> MIKQ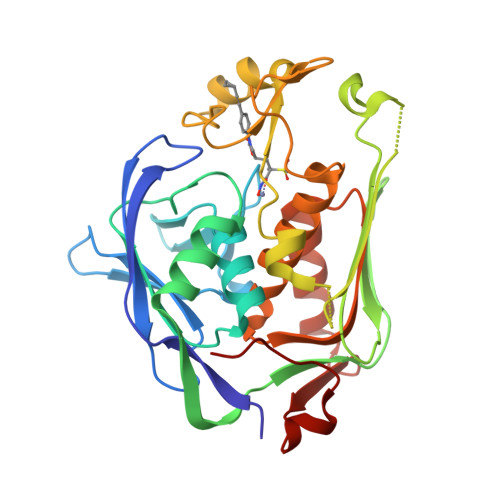RTLKNIIRATGVGLHSGEKVYLTLKPAPVDTGIVFCRTDLDPVVEIPARAENVGETTMSTTLVKGDVKVDTVEHLLSAMAGLGIDNAYVELSASEVPIMDGSAGPFVFLIQSAGLQEQEAAKKFIRIKREVSVEEGDKRAVFVPFDGFKVSFEIDFDHPVFRGRTQQASVDFSSTSFVKEVSRARTFGFMRDIEYLRSQNLALGGSVENAIVVDENRVLNEDGLRYEDEFVKHKILDAIGDLYLLGNSLIGEFRGFKSGHALNNQLLRTLIADKDAWEVVTFEDARTAPISYMRP>PVDVSVSIFINKIYGVNTLEQTYKVDGYIVAQ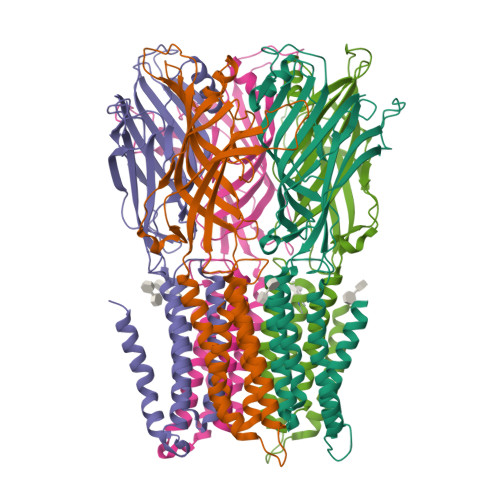WTGKPRKTPGDKPLIVENTQIERWINNGLWVPALEFINVVGSPDTGNKRLMLFPDGRVIYNARFLGSFSNDMDFRLFPFDRQQFVLELEPFSYNNQQQRFSDIQVYTENADNEEIDEWWIRGKASTHISDIRYDHLSSVQPNQNEFSRITVRIDAVRNPSYYLWSFILPLGLIIAASWSVFWLESFSERLQTSFTLMLTVVAYAFYTSNILPRLPYTTVIDQMIIAGYGSIFAAILLIIFAHHRQANGVEDDLLIQRCRLAFPLGFLAIGCVLVI[10x]>MTSAEMTSPNNNSEHQAIAKMRTMIEGFDDISHGGLPIGRSTLVSGTSGTGKTLFSIQFLYNGIIEFDEPGVFVTFEETPQDII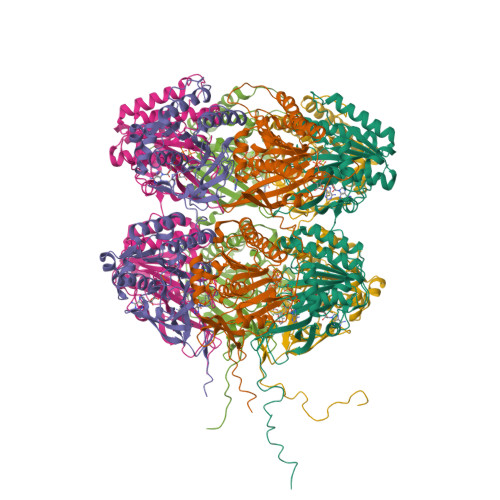KNARSFGWDLAKLVDEGKLFILDASPDPEGQEVVGGFDLSALIERINYAIQKYRARRVSIDSVTSVFQQYDASSVVRRELFRLVARLKQIGATTVMTTERIEEYGPIARYGVEEFVSDNVVILRNVLEGERRRRTLEILKLRGTSHMKGEYPFTITDHGINIFPLGAMRLTQRSSNVRVSSGVVRLDEMCGGGFFKDSIILATGATGTGKTLLVSRFVENACANKERAILFAYEESRAQLLRNAYSWGMDFEEMERQNLLKIVCAYPESAGLEDHLQIIKSEINDFKPARIAIDSLSALARGVSNNAFRQFVIGVTGYAKQEEITGLFTNTSDQFMGAHSIADSHISAITDTIILLQYVEIRGEMSRAINVFKMRGSWHDKAIREFMISDKGPDIKDSFRNFERIISGSPTRITVDEKSELSRIVRGVQEKGPES[6x]>[2x]TMAHHHHHHVTNSTDGRADGRLRVVVLGSTGSIGTQALQVIADNPDRFEVVGLAAGGAHLDTLLRQRAQTGVTNIAVADEHAAQRVGDIPYHGSDAATRLVEQTEADVVLNALVGALGLRPTLAALKTGARLALANKESLVAGGSLVLRAARPGQIVPVDSEHSALAQCLRGGTPDEVAKLVLTASGGPFRGWS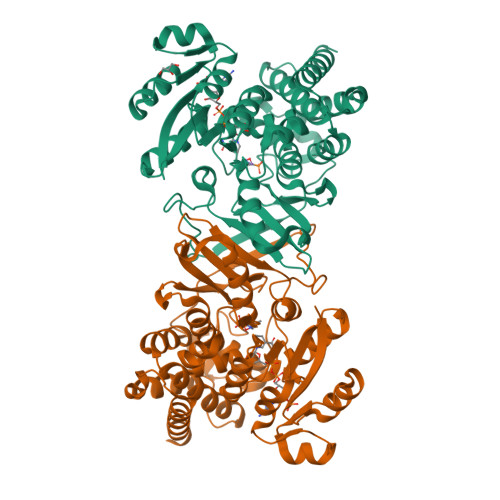AADLEHVTPEQAGAHPTWSMGPMNTLNSASLVNKGLEVIETHLLFGIPYDRIDVVVHPQSIIHSMVTFIDGSTIAQASPPDMKLPISLALGWPRRVSGAAAACDFHTASSWEFEPLDTDVFPAVELARQAGVAGGCMTAVYNAANEEAAAAFLAGRIGFPAIVGIIADVLHAADQWAVEPATVDDVLDAQRWARERAQRAVSGM>MGIKDSKINIYYGKNYPFLCRTVFNIYQNNIKKKTANNLNDKKIKEICVNFINDKTVVEDIKVEFVRNTVSDQTRKNTNTNNSVTSSDKIFAINLDFLLKTNLYYFTSYRENINRNIITNVFFQAQYNEWIDFLRNKDIEKNIIPICEHINKHLYLNTFLSFHYLTLSDIYIYYEMHKYFSGNITTN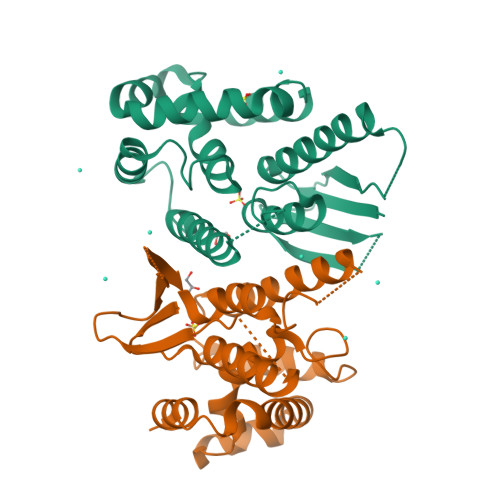LKYPKQYKNINRWFRLIKALLHDHVATDAELIQNLKVKEKIFIDGGSSGLVPRGSSHHHHHH[5x]5-[(E)-(3-carboxy-4-oxidanyl-phenyl)diazenyl]-2-oxidanyl-benzoic 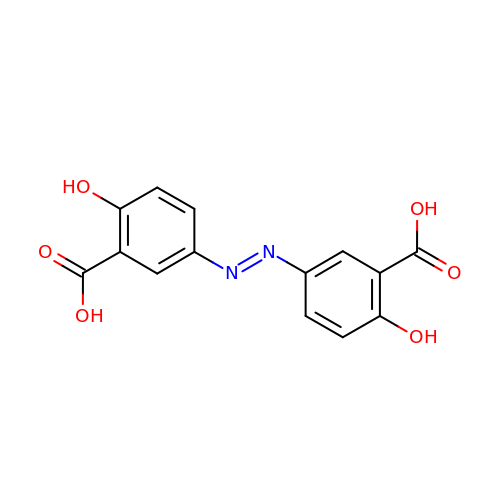acid | C14 H10 N2 O6 | QQBDLJCYGRGAKP-FOCLMDBBSA-N> MSMLKREDWYDLTRTTNWTPKYVTENELFPEEMSGARGISMEAWEKYDEPYKITYPEYVSIQREKDSGAYSIKAALERDGFVDRADPGWVSTMQLHFGAWALEEYAASTAEARMARFAKAPGNRNMATFGMMDENRHGQIQLYFPYANVKRSRKWDWAHKAIHTNEWAAIAARSFFDDMMMTRDSVAVSIMLTFAFETGFTNMQFLGLAADAAEAGDHTFASLISSIQTDESRHAQQGGPSLKILVENGKKDEAQQMVDVAIWRSWKLFSVLTGPIMDYYTPLESRNQSFKEFMLEWIVAQFERQLLDLGLDKPWYWDQFMQDLDETHHGMHLGVWYWRPTVWWDPAAGVSPEEREWLEEKYPGWNDTWGQCWDVITDNLVNGKPELTVPETLPTICNMCNLPIAHTPGNKWNVKDYQLEYEGRLYHFGSEADRWCFQIDPERYKNHTNLVDRFLKGEIQPADLAGALMYMSLEPGVMGDDAHDYEWVKAYQKKTNAA;> MSEQQPEALKPLKTWSHLAGNRRRPSEYEVVSTNLHYFTDNPERPWELDSNLPMQTWYKKYCFDSPLKHDDWNAFRDPDQLVYRTYNLLQDGQESYVQGLFD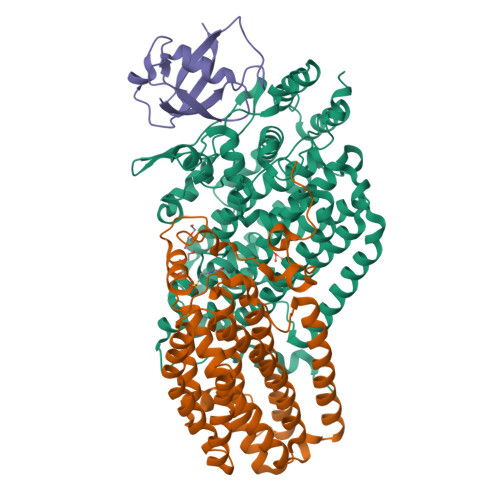QLNDRGHDQMLTREWVETLARFYTPARYLFHALQMGSVYIHQIAPASTITNCATYETADHLRWLTHTAYRTRELANCYPDVGFGKRERDVWENDPAWQGFRELIEKALIAWDWGEAFTAINLVTKPAVEEALLQQLGSLAQSEGDTLLGLLAQAQKRDAERHRRWSSALVKMALEKEGNREVLQKWVAKWEPLADKAIEAYCSALPDGENAIVEAKSASRYVRQMMGL;> MATFPIMSNFERDFVIQLVPVDTEDTMDQVAEKCAYHSINRRVHPQPEKILRVRRHEDGTLFPRGMIVSDAGLRPTETLDIIFMDN> MAAQEGVNYLSGLGLSRLICLPMALRAAIELNVFEIISQAGPDAQLSPSDIVAKIPTKNPSAAISLDRILRMLGASSILSVSTTKSGRVYGLNEESRCLVASEDKVSVVPMLLFTSDKAVVESFYNIKDVVLEEGVIPFDRTHGMDFFQYAGKEQRVNKSFNQAMGAGSTIAFDEVFEVYKGFDN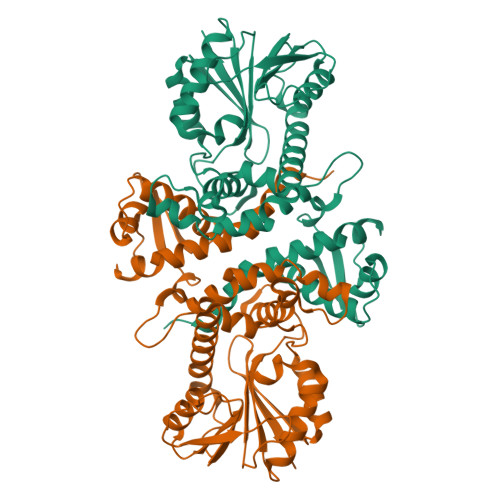LKELVDVGGGIGTSLSNIVAKYPHIRGINFELPHVIGDAPDYPGVEHVPGDMFEGVPNAQNILLKWVLHDWDDDRSIKILKNCWKALPENGTVIVIEFVLPQVLGNNAESFNALTPDLLMMALNPGGKERTTIEFDGLAKAAGFAETKFFPISQGLHVMEFHKINC3-bromophenyl hydrogen (S)-phenylphosphonate 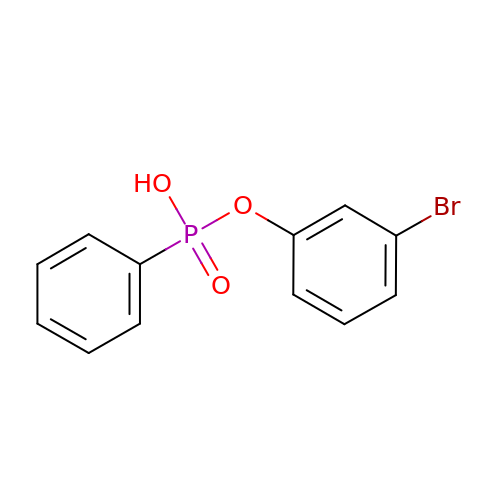| C12 H10 Br O3 P | WLHHOMQLKFZCAO-UHFFFAOYSA-N>[18x]MGRGKVKPNRKSTGDNSNVVTMIRAGSYPKVNPTPTWVRAIPFEVSVQSGIAFKVPVGSLFSANFRTDSFTSVTVMSVRAWTQLTPPVNEYSFVRLKPLFKTGDSTEEFEGRASNINTRASVGYRIPTNLRQNTVAADNVCEVRSNCRQVALVISCCF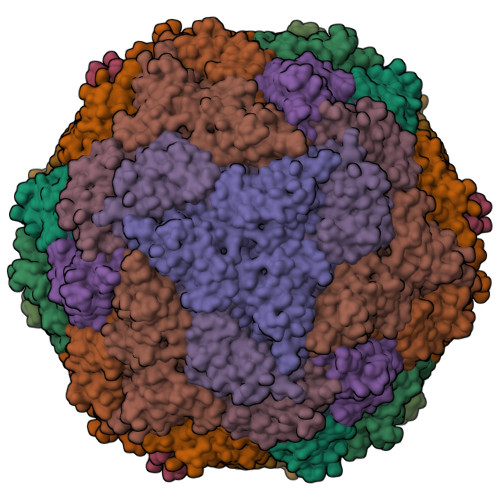N;> MGRGKVKPNRKSTGDNSNVVTMIRAGSYPKVNPTPTWVRAIPFEVSVQSGIAFKVPVGSLFSANFRTDSFTSVTVMSVRAWTQLTPPVNEYSFVRLKPLFKTGDSTEEFEGRASNINTRASVGYRIPSNLRQNTVAADNVCEVRSNCRQVALVISCCFN;> MGRGKVKPNRKSTGDNSNVVTMIRAGSYPKVNPTPTWVRAIPFEVSVQSGIAFKVPVGSLFSANFRTDSFTSVTVMSVRAWTQLTPPVNEYSFVRLKPLFKTGDSTEEFEGRASNINTRASVGYRIPTNLRQNTVAVDNVCEVRSNCRQVALVISCCFN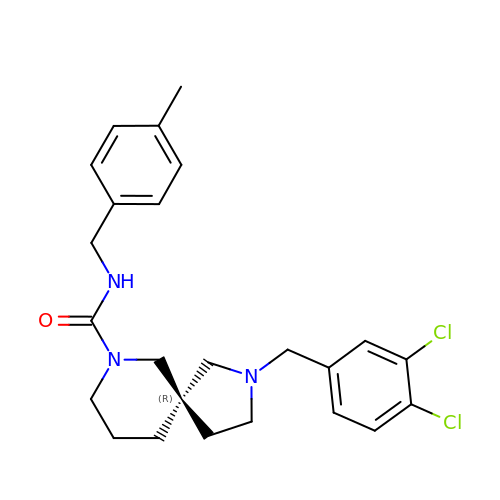(5R)-2-(3,4-dichlorobenzyl)-N-(4-methylbenzyl)-2,7-diazaspiro[4.5]decane-7-carboxamide | C24 H29 Cl2 N3 O | YFDASBFQKMHSSJ-XMMPIXPASA-N>[4x]MILVGLEAELGASKRGTDKGV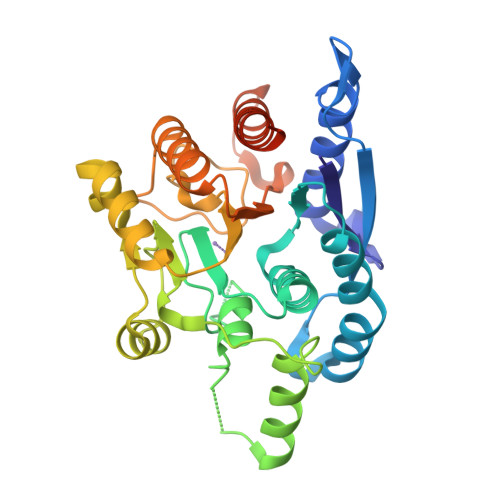RRLREALSATHGDVIKGMQTITQERCVLYKEFRYAKNFEDYYLFCKENLIPCMKEVFEKKEFPLILSSEHANMFGIFQAFRSVHKDKKIGILYLDAHADIHTAYDSDSKHIHGMPLGMVLNRVRSGFNRMSESEEKAWQKLCSLGLEKGGLEIDPKCLVYFGVRSTEQSERDVIRELQIPLFSVDAIRENMQEVVQKTKESLKAVDIIYLSLDLDIMDGKLFTSTGVRENNGLSFDELKQLLGLLLESFKDRLKAVEVTEYNPTVSIKHNNEEEKQVLEILDLIINSCKIKDKKHSFARSYLEHHHHHH>MAMSPPTQDLHIPGRLDGKVALVTGSGRGIGAAVAVHLGLLGAKVVVNYANSPTHAQKVVDEIKQLGSDAIAIKADVRQVPEIVRLFDEAVAHFGQLDIAVSNSGVVSFGHLKDVTEEEFDRVFSLNTRGQFFVAREAYKHLNNGGRIIMTSSNTSRDFSVPKHSLYSGSKGAIDSFVRIFSKDCGDKKITVNAVAPGGTVTDMFHDVSQHYIPNGETYTPEERQKMAAHASPLHRNGFPEDIARVVGFLVSAEGEWINGKVLTVDGGAAALEHHHHHH[4x]

In this study, an anthrol reductase (CbAR) from Cercospora sp. JNU001 with the ability for asymmetric reduction of various bulky substrates was identified and characterized. It belongs to the SDR superfamily and shares the highest sequence identity of 86.6% with 17β-HSDcl from Curvularia lunata. Similar to other SDRs, the overall structure of CbAR monomer contains nine α-helices and two sets of β-sheets (β1-β7), in which continuous β-sheets and seven α-helices constitute the standard Rossmann-fold motif responsible for NADPH binding and the C-terminal domain constitutes a substrate binding pocket. In both of crystal structures of CbAR-NADP+ and CbAR-NADP+-Emodin, the catalytic triad (Ser151, Tyr165 and Lys169) is well observed.

To understand the catalytic mechanism of CbAR, crystal structures of CbAR-NADP+ and CbAR-NADP+-Emodin were then solved and refined to 3.30 Å and 1.85 Å resolutions, respectively. It shows that the crystallographic asymmetric unit contains four molecules, but CbAR was eluted as a dimer in solution. Based on structure alignment, although the root mean square difference (RMSD) of superposition for the Cα atoms of crystal structures of CbAR-NADP+ and CbAR-NADP+-Emodin is 0.25Å, the regions from residue 209 to 216 are clearly different. Upon the binding of emodin, this region of CbAR-NADP+-Emodin ternary complex is visible, which is absent in the CbAR-NADP+ complex due to low electron density, indicating that this region plays a critical role in emodin recognition and binding. Ser151 plays a role in stabilizing the substrate. Tyr165 serves as a general base for proton transfer. Lys169 can not only form the hydrogen-bond interaction with NADPH but also reduce the pKa of Tyr-OH.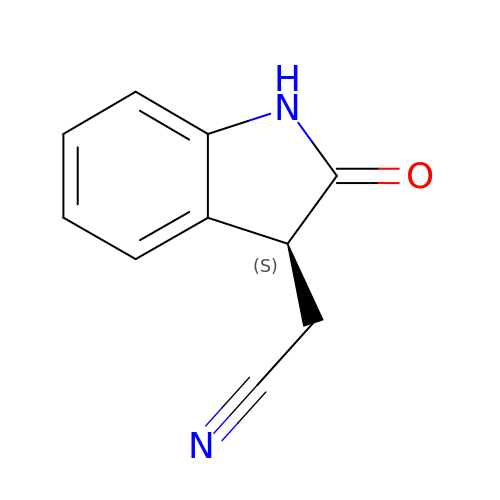[(3S)-2-oxo-2,3-dihydro-1H-indol-3-yl]acetonitrile | C10 H8 N2 O | HGYKSFCCBATMSI-QMMMGPOBSA-N>MGRDKKNTALLDMARDIG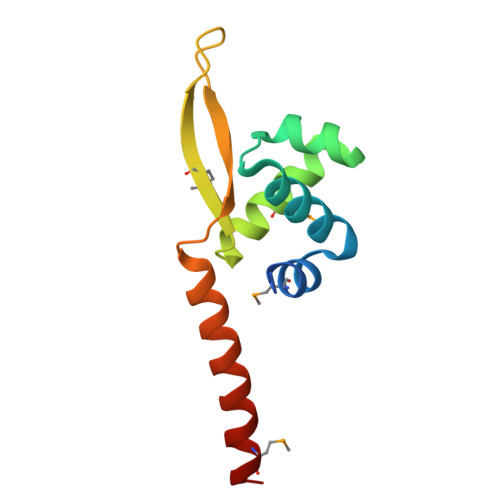GDEAVEVVKALEKKGEATDEELAELTGVRVNTVRKMLYALYDAKLATMRRVRDDETGWYYYYWRIDTKRLPEVIRTRKLQELEKLKQMLQEE[8x]>MPYNDIQHNFLKAMSDKFAEKPESTATEFYTYGGIAQKGGMRKREFIAEASKIVDSRVNSTPAYNPDAGMPQGQRYLMPYMMNHTDIMVNADDLHWINNAAMQQAWDDMKRGIVLGLDDAHGLLEARLGKEVTPDTISNYMEVLNHALPGGAVIQEHMVETKPMLVNDSYAKIFSGDDDLVDSVDRRFILDINKEFAAGYDKPGEQADQLKDAIGKKIWQILWMPTVVARQTDGGTMFRWVGMQVGMTMINAYKLCAGESVTGEFAYYAKHAAVVQLSNYMPVKRARSHNEPGGMPLGINADSTRSPALFPNDPIRAELESIAVAAMVYDQLWFGTYMSGGVGFTQYASATYTDNILEDFCYKGCEIGLDYAGGKMASIKGDKLNMDILEEIIRAENDYALTQYEAYPTVAESHFGGSVRACCAAAGCGSAVACATGLAQPALSAWSLSMLGHYERVGRLGFFGYDLQDQCTACGSYSYQSDEGMPFEMRGVNYPNYAMNVGHQSAYAGLVAGAHSANHDAWVLSPLWKVAFSDRDLPFDRGYVTREYGLGANREYTKVAGERDLIIAGHYGREPGAKL[3x];>[3x]MADEIDLYDDKGKKLAAGVPLQNISPLKNAAIKKIVNLTIRTGAVDLAGLEKKFATGAIAGRGMVIRGVNRNLPIVDKAKEIAKAVEDMLRVESGDDTNVELIAGGKRMMVQPPTARILSDYSVGLTASMGALTHAIIDVCNVSMWDAPYVHAGVWGMYPQNPDPGDGAVKMLVDIPMKNEGPGFTLRNIPVNHLAATVRKRAMQGAGLTMILEEAAQFEMGNCMGPHERGHLLDLAYEGLNANNLLYSLIKDNGQDGSLGDVIYAAVEKAKADGVIKSLKKMPSGFTVYDADDMQLWNAYACTAMLAGVCVNCASMRAGQPVPGNIMQACCLIERETGLPGPDFGMAQ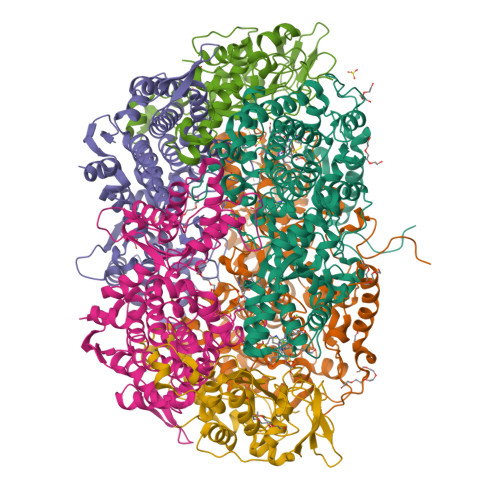GASVSSSFFSHSIYGGGGPGVFYGNHIVTRHAKGQFIPCFCAAMCIDADTMYFSPARTSALYGEVLGAIPEFAEPMRAVAEAAK;>MPQFTAGNSHVAQNRRNYMDPSYKLEKLRDIPEEDIVRLLAHRAPGEEYKSIHPPLEEMEEPDCAVRQIVKPTEGAAAGDRIRYVQYTDSMFFSPITPYQRAWEALNRYKGVDPGVLSGRTIIEARERDIEKIAKIEVDCELYDTARTGLRGRTVHGHAVRLDKDGMMFDALRRWSRGADGTVTYVKDMIGGAMDKEVTLGKPLSDAELLKKTTMYRNAQGGVWQEADDPESMDVTAQIHWKRSVGGFQPWAKMKDIKGGKKDVGVKNLKLFTPRGGVE[3x]> SGLRGTFGGNIIQHSIPAVELRQPFFPTHMGPIKLRQFHRPPLKKYSFGALSQPGPHSVQPLLKHIKKKAKMREQERQASGGGEMFFMRTPQDLTGKDGDLILAEYSEENGPLMMQVGMATKIKNYYKRKPGKDPGAPDCKYGETVYCHTSPFLGSLHPGQLLQAFENNLFRAPIYLHKMPETDFLIIRTRQGYYIRELVDIFVVGQQCPLFEVPGPNSKRANTHIRDFLQVFIYRLFWKSKDRPRRIRMEDIKKAFPSHSESSIRKRLKLCADFKRTGMDSNWWVLKSDFRLPTEEEIRAMVSPEQCCAYYSMIAAEQRLKDAGYGEKSFFAPEEENEEDFQMKIDDEVRTAPWNTTRAFIAAMKGKCLLEVTGVADPTGCGEGFSYVKIPNKPTQQKDDKEPQPVKKTVTGTDADLRRLSLKNAKQLLRKFGVPEEEIKKLSRWEVIDVVRTMSTEQARSGEGPMSKFARGSRFSVAEHQERYKEECQRIFDLQNKVLSSTEVLSTDTDSSSAEDSDFEEMGKNIENMLQNKKTSSQLSREREEQERKELQRMLLAAGSAASGNNHRDDDTASVTSLNSSATGRCLKIYRTFRDEEGKEYVRCETVRKPAVIDAYVRIRTTKDEEFIRKFALFDEQ;> SMSKSKDDAPHELESQFILRLPPEYASTVRRAVQSGHVNLKDRLTIELHPDGRHGIVRVDRVPLASKLVDLPCVMESLKTIDKKTFYKTADICQMLVSTVDGDLYPPVEEPVASTDPKASKKKDKDKEKKFIWNHGITLPLKNVRKRRFRKTAKKKYIESPDVEKEVKRLLSTDAEAVSTRWEIIAEDETKEAENQGLDISSPGMSGHRQGHDSLEHDELREIFNDLSSSSEDEDETQHQDEEDINIIDTEEDLERQLQDKLNESDEQHQENEGTNQLVMGIQKQIDNMKGKLQETQDRAKRQEDLIMKVENLALKNRFQAVLDELKQK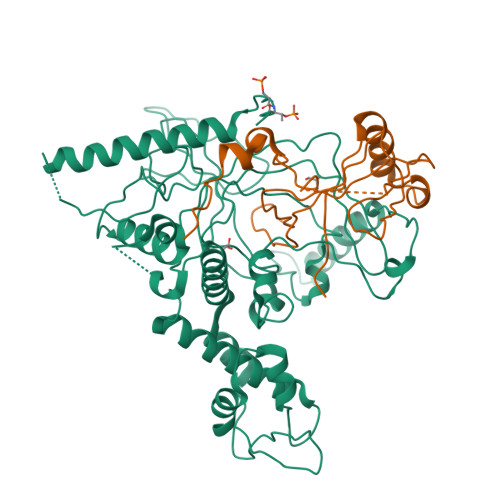EDREKEQLSSLQEELESLLEK2-[(3S)-1-[[2-[3,5-bis(chloranyl)phenyl]-6-[2-(4-methylpiperazin-4-ium-1-yl)pyrimidin-5-yl]oxy-pyridin-4-yl]methyl]pyrrolidin-1-ium-3-yl]oxyethanoic 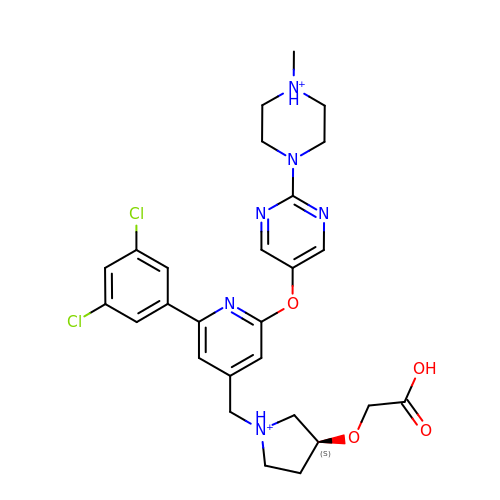acid | C27 H32 Cl2 N6 O4 | NPVPASPENGAFSC-QFIPXVFZSA-P> SLRFLY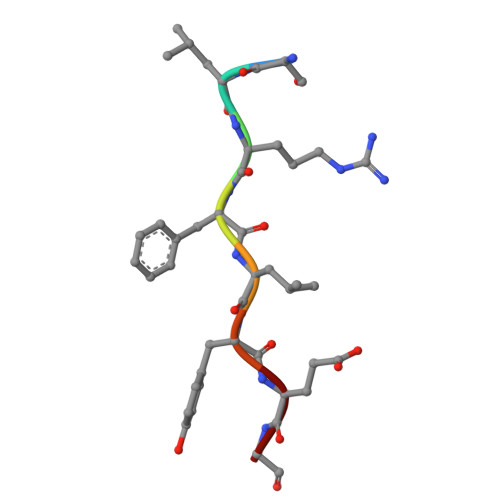EG(3~{R})-3-[(3~{R})-4-fluoranyl-1-oxidanyl-3~{H}-2,1-benzoxaborol-3-yl]-2-methylidene-butanoic acid | C12 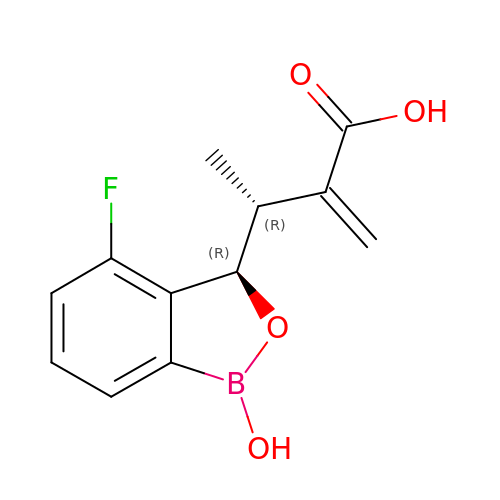H12 B F O4 | ZCBYIGIEBWTKJG-KSBSHMNSSA-N>MSEKYIVTWDMLQIHARKLASRLMPSEQWKGIIAVSRGGLVPGALLARELGIRHVDTVCISSYDHDNQRELKVLKRAEGDGEGFIVIDDLVDTGGTAVAIREMYPKAHFVTIFAKPAGRP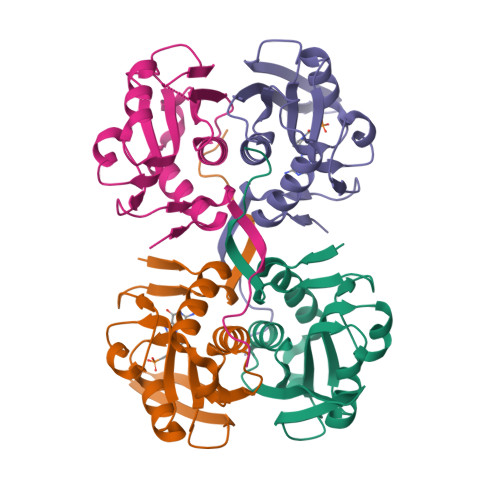LVDDYVVDIPQDTWIEQPWDMGVVFVPPISGR[4x]> MATPPLQDGAPTNGGAATKPSCGARLQNFARMAIKGPSV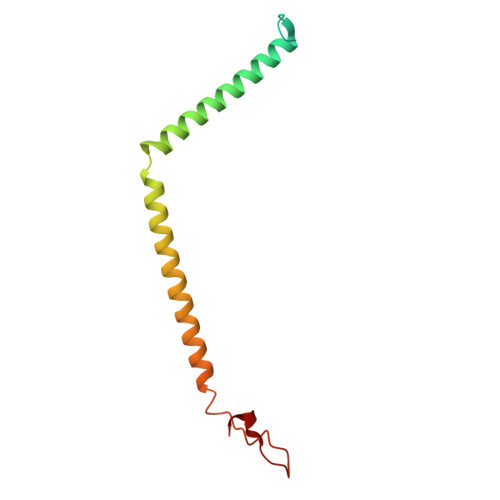PHSILFGVGAGCCAYAGYYLYRAMRLTFFDTESVALQSRLRYAEKQKLFHQELDRELAAGHIASLVAEYDPVATRLPFQPMQDRYRV>GAMGGSEFPKSRLPTLADNEIEYEKQIGKGGFGLVHKGRLVKDKSVVAIKSLILGDSEGETEMIEKFQ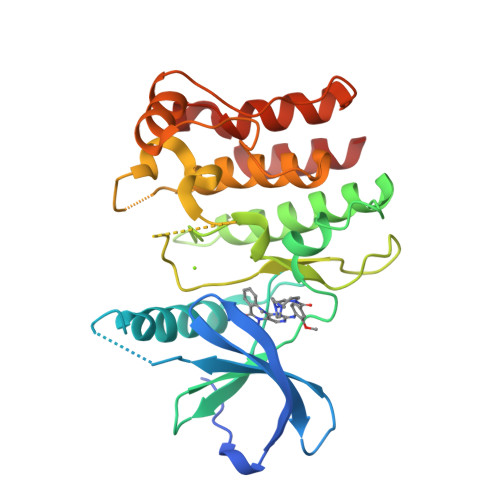EFQREVFIMSNLNHPNIVKLYGLMHNPPRMVMELVPCGDLYHRLLDKAHPIKWSVKLRLMLDIALGIEYMQNQNPPIVHRDLRSPNILLQSLDENAPVCAKVADFGLSQQSVHSVSGLLGNFQWMAPETIGAEEESYTEKADTYSFAMILYTILTGEGPFDEYSYGKIKFINMIREEGLRPTIPEDCPPRLRNVIELCWSGDPKKRPHFSYIVKELSEL[2x]>[2x]MRSRRVDVMDVMNRLILAMDLMNRDDALRVTGEVREYIDTVKIGYPLVLSEGMDIIAEF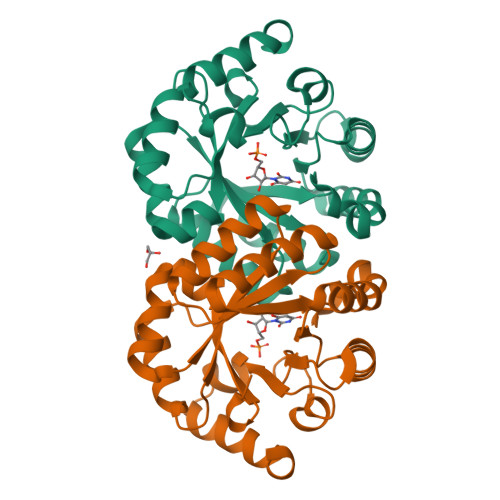RKRFGCRIIADFKVADIPETNEKICRATFKAGADAIIVHGFPGADSVRACLNVAEEMGREVFLLTEMSHPGAEMFIQGAADEIARMGVDLGVKNYVGPSTRPERLSRLREIIGQDSFLISPGVGAQGGDPGETLRFADAIIVGRSIFLADNPAAAAAGIIESIKDLLNP> EEFDPELAREVEDLRQRDQVTGLLNRPTFMVALEQAVAQAGRSEGQSGFLLIEPDHYARILPEFGLDSADALIAALAAHVASVLDDSVLAARFGEHSFALLLNGNYARTHALAETVRNAFAQHVFSVGTRSATVTVSIGGVQIGEKIASIGQVLNRGTEAVRTTAELGGNAVSIYDPAAADRAEEERIERWVEQLREALVGDGFLLHYQPVLNLQGEPLELYQAFLRLERNGEMMSPNAFMAIAEEHDLVTEIDRWVVARAIRQLGERQRAGHKTHLLVRIGPNSFSDPQMIDTIREQLAVYGVPGERLWLQTPESKVFTHLRNAQQFLAA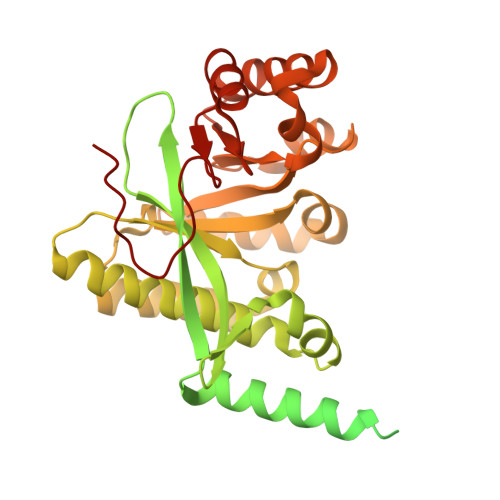VSAMDCKVGLEQFGSGLDSFQLLAHFHPAFLKLDRGITGDIASARDSQEKIREITSRAQPAGILTMAEFVADAQSMSSFFSAGVDYVQGDFVAPTGPLMNYEFG> GAMGPPQFKEIKISVAPDTPAPDAINDLLRSVDSQEVRDYCQKKGWIVIHPSNEL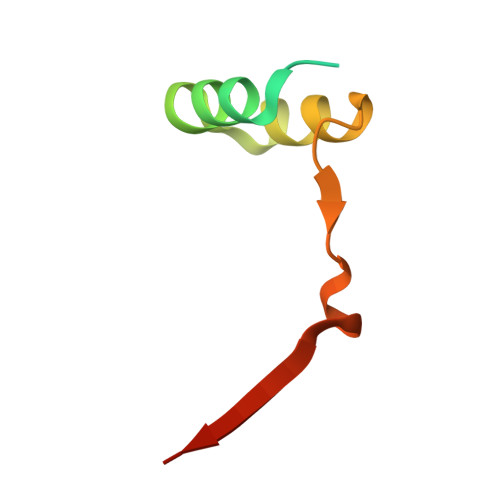VVEKHISR Endo-galactosaminidases are an underexplored family of enzymes involved in the degradation of galactosaminogalactan (GAG) and other galactosamine-containing cationic exopolysaccharides produced by fungi and bacteria. Whereas the fungal enzyme belongs to family GH114, the two bacterial enzymes do not lie in the current GH families but instead define a new family, GH191. The TIM-barrel core structure with fully conserved active-site residues and a negatively charged substrate crevice is conserved among all the families. The putative active-site residues (Asp156/Glu225 for TmGH191, Asp323/Glu391 for Env-GH191 and Asp157/Glu225 for FsGH114) overlap well with the experimentally verified nucleophile and general acid/base Asp189/Glu247 in Ega3, Asp196/Glu222 in Sph3 and Asp160/Glu223 in PelAH.

We could not detect any binding, or enzymatic cleavage of the GAG oligomers, for the T. maritima enzyme, which raises the question as to whether the T. maritima enzyme is an endo-galactosaminidase or whether GAG is not a substrate for this family. The TmGH191 crystals all showed a varying degree of twinning. The structure is composed of tightly packed trimers stacked on each other along their common pseudo-threefold axis. A pair of adjacent trimers form the asymmetric unit, with the two trimers having slightly different orientations (11.5° rotation around the common axis). The stacks of trimers pack into a sparse honeycomb-like structure with wide wells around the pseudo-63 axis and a solvent content of 82.5%. Sph3 has a rather less charged surface due to its activity on neutral GlcNAcylated GAG. A closer inspection shows that the substrate crevice is partially blocked in ‘apo’ TmGH191, especially over the active site via the loop between βi2 and βi3, with Trp121 bridging the active site and blocking access towards the putative −1 subsite. The TmGH191 crystals prepared in this study were soaked with GalN and GalNAc, and a data set was obtained for a GalN-soaked crystal. While no distinct density for a bound carbohydrate was observed, difference density in the substrate-binding crevice of TmGH191 suggests that something has bound, although it could not be conclusively modelled. Some flexibility in the side chain of Trp121 was noted when comparing the native and soaked structures.

>TEGWFMPFDNWLYQLQNADPVEISSSGFEIAVIDYSKDGSESGEYSPEEIKIMVDAGVVPVAYVNIGQAEDYRFYWKESWYTNTPEWLGEEDPAWPGNYFVKYWYNEWKEIVFSYLDRVIDQGFKGIYLDRIDSFEYWAQEGVISRRSAARKMINFVLEIAEYVRERKPDMLIIPQNGENILDFDDGQLASTVSGWAVENLFYLKTIPLEENETKSRLEYLIRLNRKGKFILSVDYVDDGSDSFENISRILDYYEKAKRNGCIPYAARSDLELDEMNVIEGIQPPEALKDYESRTYR[6x]>[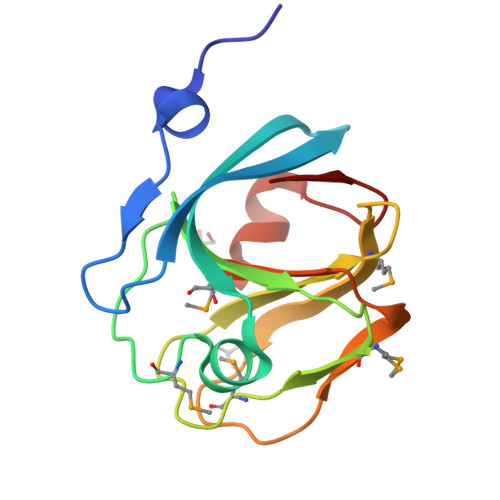2x]GGTKTAAEAAAPAVHPVSGLQIVPVTVTGTSGRHVFRSELARTSAEQAKGLMFRTELGDEEGMIFLRNPPDMATFWMRNTVIPLDIIFVGLDRRVMNIAANAVPYDETPLPAAGPTLAVLEINGGLAARLGIKPGDKVEW>[2x]XXXXXXXWDNSSPVIVQGGSLRTWSFANPAI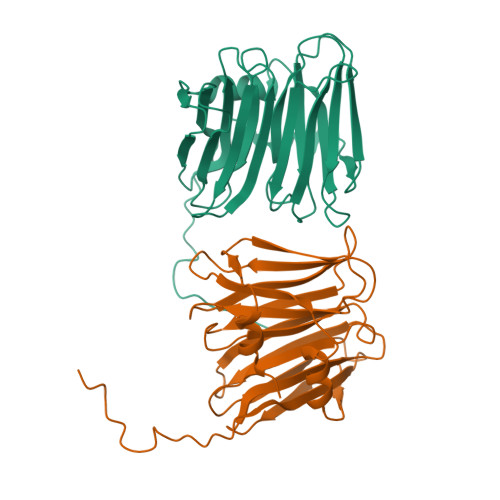ESVQVLLKTEGRPLDADVELWQGPDNTPHKMRVYVEDGALRTFNAVIGTPRGPNTVAIRNIGQLEFPLDAVVRPDRDDGLAAGIASVATRSETIQGGALRTYPFNPTVDSVAIILKTDGRPLNARIELLQGPNNNKQVVELYTEDGLDRPFFAIVETPGSGNVVRVVNTAPVEFPLYASVDAYRVGGGGDWADDGLMIGRAF> HHHHHHAVAKDSTESKSWEPFSLSPIKDPQALHKELCSKNVIPVTSTLEDLLPATQAQHVFIKRGTFHSYNWTIKGRSLNMDRLRETCQSLVDRHSILRTSFVEHEGHPIQLVLANLDVKVREVQCWPGEDPMEVCKALWDGKDWPTLNVLGGSLPVRFTLVSCPGNEHVVLTIQISHSQWDGVSIPKLFSDFAAIYNQTPLPPTSDFAHYLYHRVSSAREDVQQDPTFQFWRHYLDGAKMAVPFAPRALTLCAEPAAAAQSGQTLWTFKGIVPPTLPSGITMATLVKAATALFLSYHLGSRDVVFGHTVNGRNLPMDNIESLLGCTLNFVPLRVT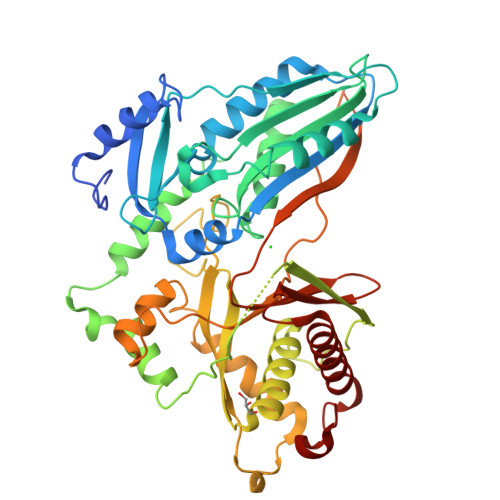FPEDSTDWTVMDLLHHTQTQYTRALSHEHVELRDIFQHSTNWPAETPLSLIVQHQNIDLSFSLPLRGSSVSGDGEDDSSLDVQYSKFARFDPLDEVWIFTEPHADRLEVQVCANSRVLGQEQATELANNISAIITKFSTDPTARLLDITF> MRGSGQFRVIGPGHPIRALVGDEAELPCRISPGKNATGMEVGWYRSPFSRVVHLYRNGKDQDAEQAPEYRGRTELLKES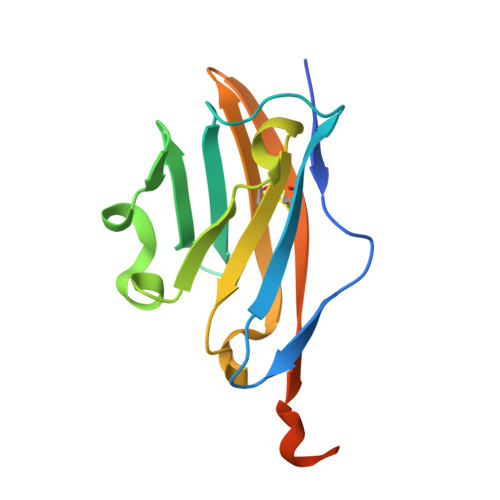IGEGKVALRIQNVRFSDEGGYTCFFRDAEYQEEAAVELKVEDPFYWINPGRSRSHHHHHH> GPHMSEAKAKAIGKVDDLLELYMGIRDIDLATTMFEAGKDKSNPDEFAVALDETLGDFAFPDE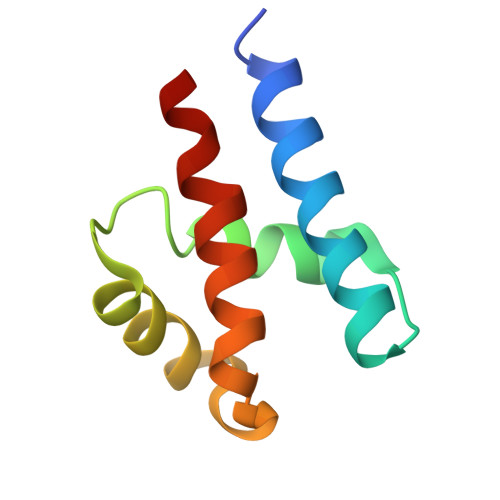FLFDVWGAISDMKQGR> MLANENSLLTMFRELGSGKLPLQIEQFERGKTIFFPGDPAERVYLLVKGAVKLSRVYESGEEITVALLRENSVFGVLSLLT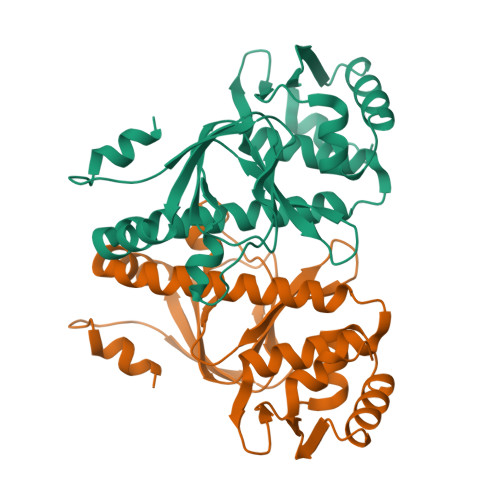GQRSDRFYHAVAFTPVQLFSVPIEFMQKALIERPELANVMLQGLSSRILQTEMMIETLAHRDMGSRLVSFLLILCRDFGIPSPDGITIDLKLSHQAIAEAIGSTRVTVTRLLGDLRESKLIAIHKKRITVFNPVALSQQFS> MEFPIGSLETNNFRRFTPESLVEIEKQIAAKQGTKKAREKHREQKDQEEKPRPQLDLKACNQLPKFYGELPAELIGEPLEDLDPFYSTHRTFMVLNKGRTISRFSATRALWLFSPFNLIRRTAIKVSVHSWFSLFITVTILVNCVCMTRTDLPEKIEYVFTVIYTFEALIKILARGFCLNEFTYLRDPWNWLDFSVITLAYVGTAIDLRGISGLRTFRVLRALKTVSVIPGLKVIVGALIHSVKKLADVTILTIFCLSVFALVGLQLFKGNLKNKCVKNDMAVNETTNYSSHRKPDIYINKRGTSDPLLCGNGSDSGHCPDGYICLKTSDNPDFNYTSFDSFAWAFLSLFRLMTQDSWERLYQQTLRTSGKIYMIFFVLVIFLGSFYLVNLILAVVTMAYEEQNQATTDEIEAKEKKFQEALEMLRKEQEVLAALGIDTTSLHSHNGSPLTSKNASERRHRIKPRVSEGSTEDNKSPRSDPYNQRRMSFLGLASGKRRASHGSVFHFRSPGRDISLPEGVTDDGVFPGDHESHRGSLLLGGGAGQQGPLPRSPLPQPSNPDSRHGEDEHQPPPTSELAPGAVDVSAFDAGQKKTFLSAEYLDEPFRAQRAMSVVSIITSVLEELEESEQKCPPCLTSLSQKYLIWDCCPMWVKLKTILFGLVTDPFAELTITLCIVVNTIFMAMEHHGMSPTFEAMLQIGNIVFTIFFTAEMVFKIIAFDPYYYFQKKWNIFDCIIVTVSLLELGVAKKGSLSVLRSFRLLRVFKLAKSWPTLNTLIKIIGNSVGALGNLTIILAIIVFVFALVGKQLLGENYRNNRKNISAPHEDWPRWHMHDFFHSFLIVFRILCGEWIENMWACMEVGQKSICLILFLTVMVLGNLVVLNLFIALLLNSFFADNLTAPEDDGEVNNLQVALARIQVFGHRTKQALCSFFSRSCPFPQPKAEPELVVKLPLSSSKAENHIAANTARGSSGGLQAPRGPRDEHSDFIANPTVWVSVPIAEGESDLDDLEDDGGEDAQSFQQEVIPKGQQEQLQQVERCGDHLTPRSPGTGTSSEDLAPSLGETWKDESVPQVPAEGVDDTSSSEGSTVDCLDPEEILRKIPELADDLEEPDDCFTEGCIRHCPCCKLDTTKSPWDVGWQVRKTCYRIVEHSWFESFIIFMILLSSGSLAFEDYYLDQKPTVKALLEYTDRVFTFIFVFEMLLKWVAYGFKKYFTNAWCWLDFLIVNISLISLTAKILEYSEVAPIKALRTLRALRPLRALSRFEGMRVVVDALVGAIPSIMNVLLVCLIFWLIFSIMGVNLFAGKFWRCINYTDGEFSLVPLSIVNNKSDCKIQNSTGSFFWVNVKVNFDNVAMGYLALLQVATFKGWMDIMYAAVDSREVNMQPKWEDNVYMYLYFVIFIIFGGFFTLNLFVGVIIDNFNQQKKKLGGQDIFMTEEQKKYYNAMKKLGSKKPQKPIPRP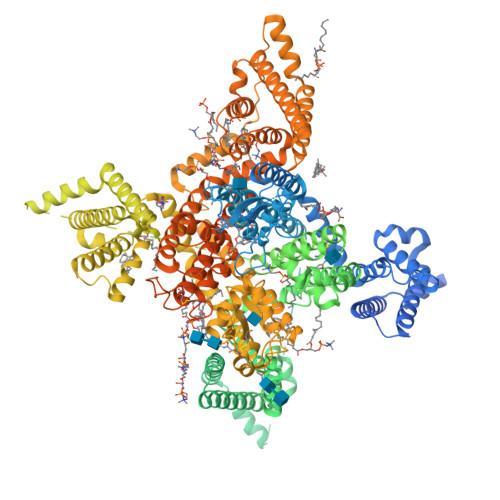LNKFQGFVFDIVTRQAFDITIMVLICLNMITMMVETDDQSEEKTKILGKINQFFVAVFTGECVMKMFALRQYYFTNGWNVFDFIVVVLSIASLIFSAILKSLQSYFSPTLFRVIRLARIGRILRLIRAAKGIRTLLFALMMSLPALFNIGLLLFLVMFIYSIFGMSSFPHVRWEAGIDDMFNFQTFANSMLCLFQITTSAGWDGLLSPILNTGPPYCDPNLPNSNGTRGDCGSPAVGIIFFTTYIIISFLIMVNMYIAVILENFNVATEESTEPLSEDDFDMFYETWEKFDPEATQFITFSALSDFADTLSGPLRIPKPNRNILIQMDLPLVPGDKIHCLDILFAFTKNVLGESGELDSLKANMEEKFMATNLSKSSYEPIATTLRWKQEDISATVIQKAYRSYVLHRSMALSNTPCVPRAEEEAASLPDEGFVAFTANENCVLPDKSETASATSFPPSYESVTRGLSDRVNMRTSSSIQNEDEATSMELIAPGP>[2x]EGPALYEDPPDHKTSPSGKPATLKICSWNVDGLRAWIKKKGLDWVKEEAPDILCLQETKCSENKLPAELQELPGLSHQYWSAPSDKEGYSGVGLLSRQCPLKVSYGIGDEEHDQEGRVIVAEFDSFVLVTAYVPNAGRGLVRLEYRQRWDEAFRKFLKGLASRKPLVLCGDLNVAHEEIDLRNPKGNKKNAGFTPQERQGFGELLQAVPLADSFRHLYPNTPYAYTFWTYMMNARSKN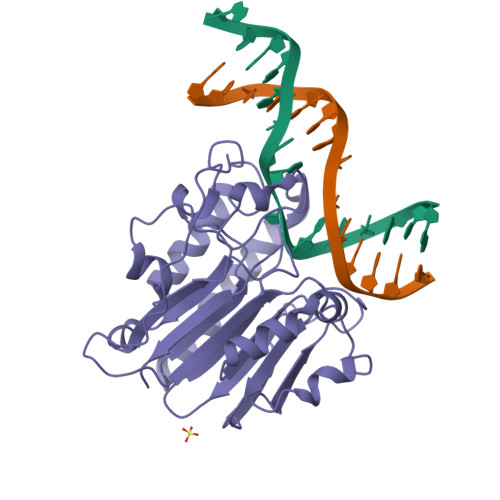VGWRLDYFLLSHSLLPALCDSKIRSKALGSDHCPITLYLAL> MAVTDLSLTNSSLMPTLNPMIQQLALAIAASWQSLPLKPYQLPEDLG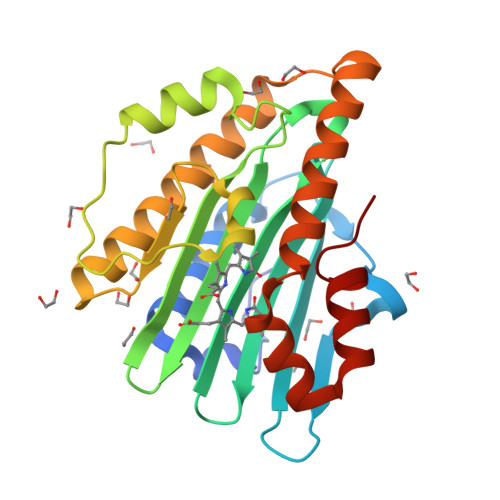YVEGRLEGEKLVIENRCYQTPQFRKMHLELAKVGKGLDILQCVMFPEPLYGLPLFGCDIVAGPGGVSAAIADLSPTQSDRQLPAAYQKSLAELGQPEFEQQRELPPWGEIFSEYCLFIRPSNVTEEERFVQRVVDFLQIHCHQSIVAEPLSEAQTLEHRQGQIHYCQQQQKNDKTRRVLEKAFGEAWAERYMSQVLFDVIQ> MTTDLNAPQLVVDDYEQLIIDSLVHTNVVSNGEFTDLDASGFMRPFAGTMAYAGSELLYKANLASIAAAKSFFKNVLGVPEDTGTKATTTLQFGLSASLSTDFIVPINFQVSDLSGTLRFYTIGNLVIPAGATFGTIEAIAEDIGEKYNVSANFIDQYSTPLTYLQYVTN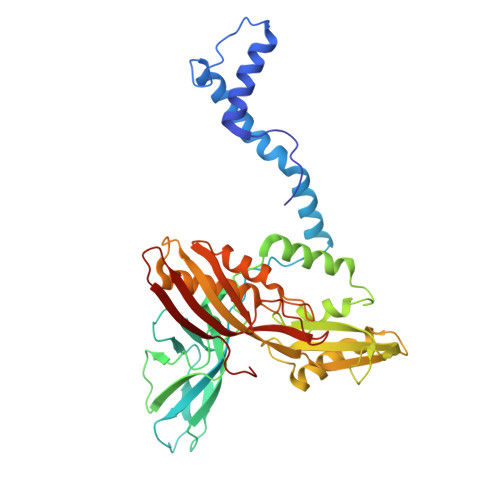IRPATNGRSGETIDNLIERCAQIIRIRNPVSALDFEQLAELTMGEGSRCKAIGLLGINKIVTDPQPGVVHLFLLDVNGNPADPVTISTVGATLQPRIMLGTRLLISPMEVLNIELELIALSDSSKTFQQLADDILEALKVFFNPANLTPGEPVLIEEVKFAIRSVGGLSISYLQMNDNAINIPMPNQWTIPRFSYIGFELTDSEGTVYRDNVVTVTNPEE> NEKLAKKKIVSIDAGRKYFSPEQLKEIIDKAKHYGYTDLHLLVGNDGLRFMLDDMSITANGKTYASDDVKRAIEKGTNDYYNDPNGNHLTESQMTDLINYAKDKGIGLIPTVNSPGHMDAILNAMKELGIQNPNFSY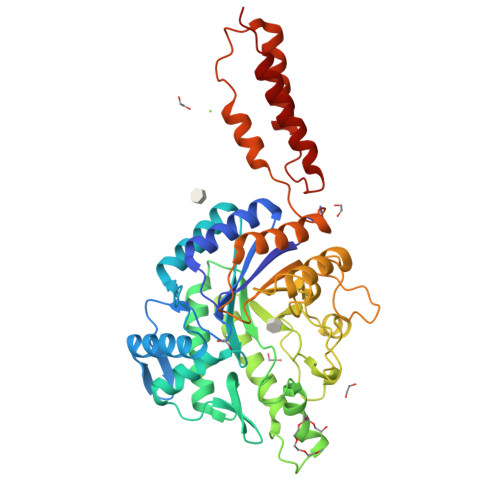FGKKSARTVDLDNEQAVAFTKALIDKYAAYFAKKTEIFNIGLDEYANDATDAKGWSVLQADKYYPNEGYPVKGYEKFIAYANDLARIVKSHGLKPMAFNDGIYYNSDTSFGSFDKDIIVSMWTGGWGGYDVASSKLLAEKGHQILNTNDAWYYVLGRNADGQGWYNLDQGLNGIKNTPITSVPKTEGADIPIIGGMVAAWADTPSARYSPSRLFKLMRHFANANAEYFAADYESAEQALNEVPKDLNRYTAESVTAVKEAEKAIRSLDSNLSRAQQDTIDQAIAKLQETVNNLTLT> AISIKTPEDIEKMRVAGRLAAEVLEMIEPYVKPGVSTGELDRICNDYIVNEQHAVSACLGYHGYPKSVCISINEVVCHGIPDDAKLLKDGDIVNIDVTVIKDGFHGDTSKMFIVGKPTIMGERLCR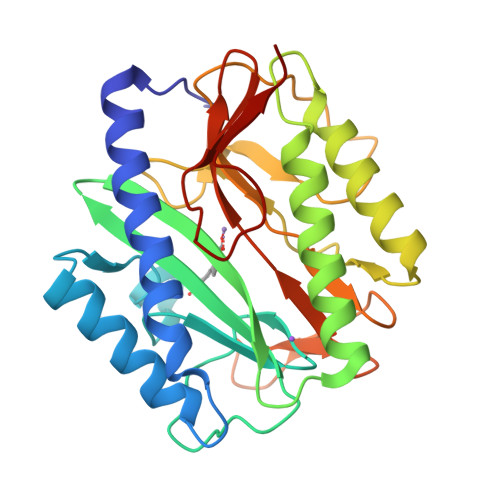ITQESLYLALRMVKPGINLREIGAAIQKFVEAEGFSVVREYCGHGIGRGFHEEPQVLHYDSRETNVVLKPGMTFTIEPMVNAGKKEIRTMKDGWTVKTKDRSLSAQYEHTIVVTDNGCEILTLRKDDTIPAIISHD>MLLKNAVQLICYPDRIGNNLKDLYTVVDTHLSEAIGGLHILPFFPSNADGGFSPLTHKEVDPKVGTWDDIEAFTAKYDLCVDLTVNHISDESPEFTDFIANGFDSEYADLFVHVDKFGEISPDDMAKIHIRKEKEPFREVTLSDGTKTRVWCTFTEQQIDLNYESDLAYQLMESYIGFLTSKGVNLLRLDAFGYTTKRIGTSCFLVEPEVYQILDWVNQVALKHGAECLPEVH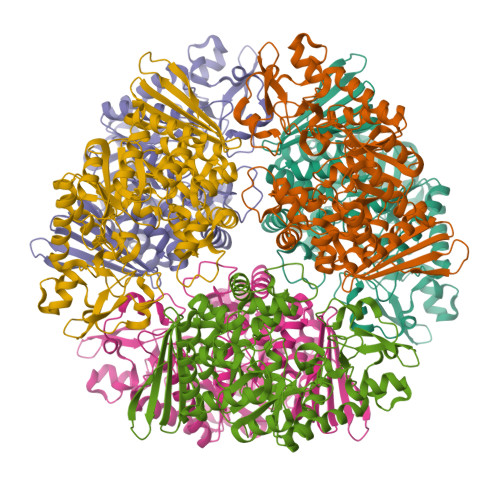DHTSYQYAISRRNMHPYGFALPPLLLYSLLDANSTYLKNWLRMCPRNMVTVLDTHDGICIPDVEGVLPDEKIKVLIDNIDARSADPIMRRSAANIHSVGAIYQLTCTFYDALMQNDDAYIAARAIQFFTPGIPQVYYVGLLAGCNDHELMEQSGELRDINRHYYTLEEVEQDIQKPVVQRLLSLMKFRSNYPAFDGHFELNYSNNSSVAMAWRHGDYYCHLFVDLNFKTVKVTYTDVETGETRHLEC[18x]5-methyl-~{N}-[2,2,2-tris(fluoranyl)ethyl]-1,2-oxazole-3-carboxamide 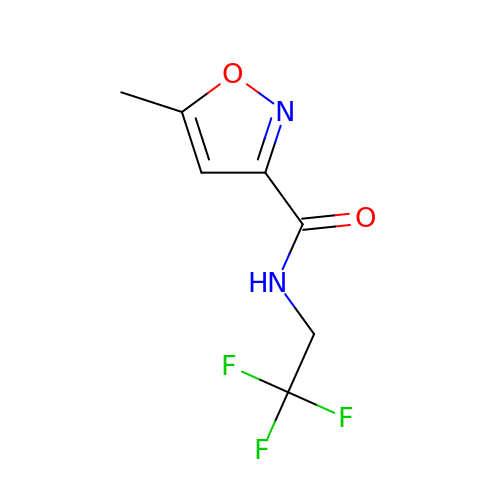| C7 H7 F3 N2 O2 | XCSPVFNSKGQNKR-UHFFFAOYSA-N>[2x]SNLVDNTNQVEVLQRDPNSPLYSVKSFEELRLKPQLLQGVYAMGFNRPSKIQENALPLMLAEPPQNLIAQSQSGTGKTAAFVLAMLSQVEPANKYPQCLCLSPTYELALQTGKVIEQMGKFYPELKLAYAVRGNKLERGQKISEQIVIGTPGTVLDWCSKLKFIDPKKIKVFVLDEADVMIATQGHQDQSIRIQRMLPRNCQMLLFSATFEDSVWKFAQKVVPDPN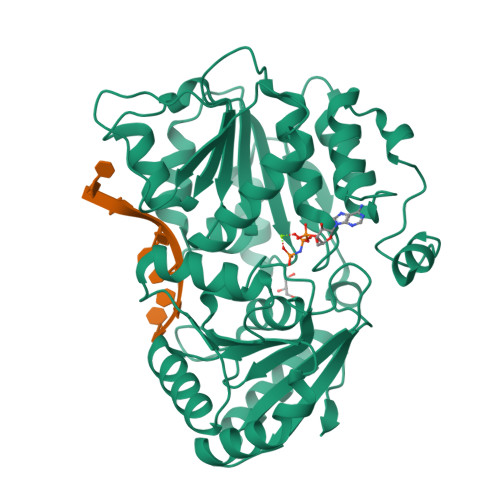VIKLKREEETLDTIKQYYVLCSSRDEKFQALCNLYGAITIAQAMIFCHTRKTASWLAAELSKEGHQVALLSGEMMVEQRAAVIERFREGKEKVLVTTNVCARGIDVEQVSVVINFDLPVDKDGNPDNETYLHRIGRTGRFGKRGLAVNMVDSKHSMNILNRIQEHFNKKIERLDTDDLDEIEKIAN> TGRPEWIWLALGTALMGLGTLYFLVKGMGVSDPDAKKFYAITTLVPAIAFTMYLSMLLGYGLTMVPFGGEQNPIYWARYADWLFTTPLLLLDLALLVDADQGTILALVGADGIM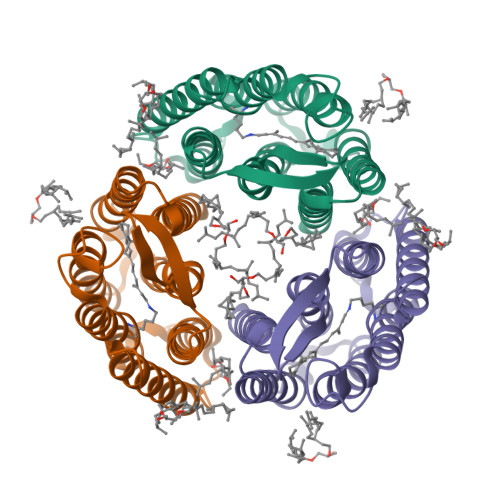IGTGLVGALTKVYSYRFVWWAISTAAMLYILYVLFFGFTSKAESMRPEVASTFKVLRNVTVVLWSAYPVVWLIGSEGAGIVPLNIETLLFMVLDVSAKVGFGLILLRSRAIFGEA> MSANSPTGNDPHVFGIPVNATPSNMGSPGSPVNVPPPMNPAVANVNHPVMRTNSNSNANEGTRTLTREQIQQLQQRQRLLLQQRLLEQQRKQQALQNYEAQFYQMLMTLNKRPKRLYNFVEDADSILKKYEQYLHSFEFHIYENNYKICAPANSRLQQQQKQPELTSDGLILTKNNETLKEFLEYVARGRIPDAIMEVLRDCNIQFYEGNLILQVYDHTNTVDVTPKENKPNLNSSSSPSNNNSTQDNSKIQQPSEPNSGVANTGANTANKKASFKRPRVYRTLLKPNDLTTYYDMMSYADNARFSDSIYQQFESEILTLTKRNLSLSVPLNPYEHRDMLEETAFSEPHWDSEKKSFIHEHRAESTREGTKGVVGHIEERDEFPQHSSNYEQLMLIMNERTTTITNSTFAVSLTKNAMEIASSSSNGVRGASSSTSNSASNTRNNSLANGNQVALAAAAAAAAVGSTMGNDNNQFSRLKFIEQWRINKEKRKQQALSANINPTPFNARISMTAPLTPQQQLLQRQQQALEQQQNGGAMKNANKRSGNNATSNNNNNNNNLDKPKVKRPRKNAKKSESGTPAPKKKRMTKKKQSASSTPSSTTMS;> MSSNPENSGVNANNNTGTGNADAITGAQQNMVLQPRQLQEMAAKFRTLLTEARNVGETTPRGKELMFQAAKIKQVYDALTLNRRRQQAAQAYNNTSNSNSSNPASIPTENVPNSSQQQQQQQQQTRNNSNKFSNMIKQVLTPEENQEYEKLWQNFQVRHTSIKEKETYLKQNIDRLEQEINKQTDEGPKQQLQEKKIELLNDWKVLKIEYTKLFNNYQNSKKTFYVECARHNPALHKFLQESTQQQRVQQQRVQQQQQQQQQQQQQQQQQQQQQQQRQGQNQRKISSSNSTEIPSVTGPDALKSQQQQQNTITATNNPRGNVNTSQTEQSKAKVTNVNATASMLNNISSSKSAIFKQTEPAIPISENISTKTPAPVAYRSNRPTITGGSAMNASALNTPATTKLPPYEMDTQRVMSKRKLRELVKTVGIDEGDGETVIDGDVEELLLDLADDFVTNVTAFSCRLAKHRKSDNLEARDIQLHLERNWNIRIPGYSADEIRSTRKWNPSQNYNQKLQSITSDKVAAAKNNGNNVASLNTKK;> MSLTEQIEQFASRFRDDDATLQSRYSTLSELYDIMELLNSPEDYHFFLQAVIPLLLNQLKEVPISYDAHSPEQKLRNSMLDIFNRCLMNQTFQPYAMEVLEFLLSVLPKENEENGILCMKVLTTLFKSFKSILQDKLDSFIRIIIQIYKNTPNLINQTFYEAGKAEQGDLDSPKEPQADELLDEFSKNDEEKDFPSKQSSTEPRFENSTSSNGLRSSMFSFKILSECPITMVTLYSSYKQLTSTSLPEFTPLIMNLLNIQIKQQQEAREQAESRGEHFTSISTEIINRPAYCDFILAQIKATSFLAYVFIRGYAPEFLQDYVNFVPDLIIRLLQDCPSELSSARKELLHATRHILSTNYKKLF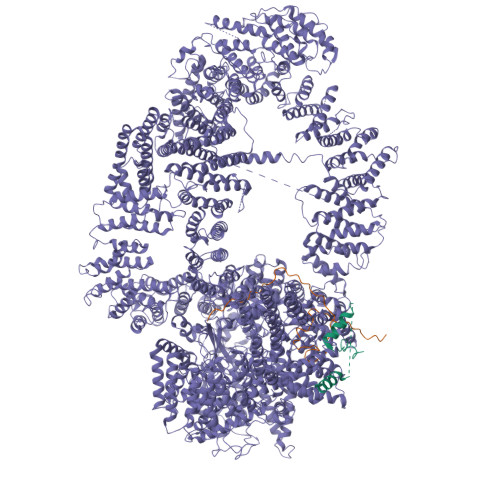LPKLDYLFDERILIGNGFTMHETLRPLAYSTVADFIHNIRSELQLSEIEKTIKIYTGYLLDESLALTVQIMSAKLLLNLVERILKLGKENPQEAPRAKKLLMIIIDSYMNRFKTLNRQYDTIMKYYGRYETHKKEKAEKLKNSIQDNDKESEEFMRKVLEPSDDDHLMPQPKKEDINDSPDVEMTESDKVVKNDVEMFDIKNYAPILLLPTPTNDPIKDAFYLYRTLMSFLKTIIHDLKVFNPPPNEYTVANPKLWASVSRVFSYEEVIVFKDLFHECIIGLKFFKDHNEKLSPETTKKHFDISMPSLPVSATKDARELMDYLAFMFMQMDNATFNEIIEQELPFVYERMLEDSGLLHVAQSFLTSEITSPNFAGILLRFLKGKLKDLGNVDFNTSNVLIRLFKLSFMSVNLFPNINEVVLLPHLNDLILNSLKYSTTAEEPLVYFYLIRTLFRSIGGGRFENLYRSIKPILQVLLQSLNQMILTARLPHERELYVELCITVPVRLSVLAPYLPFLMKPLVFALQQYPDLVSQGLRTLELCIDNLTAEYFDPIIEPVIDDVSKALFNLLQPQPFNHAISHNVVRILGKLGGRNRQFLKPPTDLTEKTELDIDAIADFKINGMPEDVPLSVTPGIQSALNILQSYKSDIHYRKSAYKYLTCVLLLMTKSSAEFPTNYTELLKTAVNSIKLERIGIEKNFDLEPTVNKRDYSNQENLFLRLLESVFYATSIKELKDDAMDLLNNLLDHFCLLQVNTTLLNKRNYNGTFNIDLKNPNFMLDSSLILDAIPFALSYYIPEVREVGVLAYKRIYEKSCLIYGEELALSHSFIPELAKQFIHLCYDETYYNKRGGVLGIKVLIDNVKSSSVFLKKYQYNLANGLLFVLKDTQSEAPSAITDSAEKLLIDLLSITFADVKEEDLGNKVLENTLTDIVCELSNANPKVRNACQKSLHTISNLTGIPIVKLMDHSKQFLLSPIFAKPLRALPFTMQIGNVDAITFCLSLPNTFLTFNEELFRLLQESIVLADAEDESLSTNIQKTTEYSTSEQLVQLRIACIKLLAIALKNEEFATAQQGNIRIRILAVFFKTMLKTSPEIINTTYEALKGSLAENSKLPKELLQNGLKPLLMNLSDHQKLTVPGLDALSKLLELLIAYFKVEIGRKLLDHLTAWCRVEVLDTLFGQDLAEQMPTKIIVSIINIFHLLPPQADMFLNDLLLKVMLLERKLRLQLDSPFRTPLARYLNRFHNPVTEYFKKNMTLRQLVLFMCNIVQRPEAKELAEDFEKELDNFYDFYISNIPKNQVRVVSFFTNMVDLFNTMVITNGDEWLKKKGNMILKLKDMLNLTLKTIKENSFYIDHLQLNQSIAKFQALYLRFTELSERDQNPLLLDFIDFSFSNGIKASYSLKKFIFHNIIASSNKEKQNNFINDATLFVLSDKCLDARIFVLKNVINSTLIYEVATSGSLKSYLVEDKKPKWLELLHNKIWKNSNAILAYDVLDHHDLFRFELLQLSAIFIKADPEIIAEIKKDIIKFCWNFIKLEDTLIKQSAYLVTSYFISKFDFPIKVVTQVFVALLRSSHVEARYLVKQSLDVLTPVLHERMNAAGTPDTWINWVKRVMVENSSSQNNILYQFLISHPDLFFNSRDLFISNIIHHMNKITFMSNSNSDSHTLAIDLASLILYWENKTLEITNVNNTKTDSDGDVVMSDSKSDINPVEADTTAIIVDANNNSPISLHLREACTAFLIRYVCASNHRAIETELGLRAINILSELISDKHWTNVNVKLVYFEKFLIFQDLDSENILYYCMNALDVLYVFFKNKTKEWIMENLPTIQNLLEKCIKSDHHDVQEALQKVLQVIMKAIKAQGVSVIIEEESPGKTFIQMLTSVITQDLQETSSVTAGVTLAWVLFMNFPDNIVPLLTPLMKTFSKLCKDHLSISQPKDAMALEEARITTKLLEKVLYILSLKVSLLGDSRRPFLSTVALLIDHSMDQNFLRKIVNMSRSWIFNTEIFPTVKEKAAILTKMLAFEIRGEPSLSKLFYEIVLKLFDQEHFNNTEITVRMEQPFLVGTRVEDIGIRKRFMTILDNSLERDIKERLYYVIRDQNWEFIADYPWLNQALQLLYGSFNREKELSLKNIYCLSPPSILQEYLPENAEMVTEVNDLELSNFVKGHIASMQGLCRIISSDFIDSLIEIFYQDPKAIHRAWVTLFPQVYKSIPKNEKYGFVRSIITLLSKPYHTRQISSRTNVINMLLDSISKIESLELPPHLVKYLAISYNAWYQSINILESIQSNTSIDNTKIIEANEDALLELYVNLQEEDMFYGLWRRRAKYTETNIGLSYEQIGLWDKAQQLYEVAQVKARSGALPYSQSEYALWEDNWIQCAEKLQHWDVLTELAKHEGFTDLLLECGWRVADWNSDRDALEQSVKSVMDVPTPRRQMFKTFLALQNFAESRKGDQEVRKLCDEGIQLSLIKWVSLPIRYTPAHKWLLHGFQQYMEFLEATQIYANLHTTTVQNLDSKAQEIKRILQAWRDRLPNTWDDVNMWNDLVTWRQHAFQVINNAYLPLIPALQQSNSNSNINTHAYRGYHEIAWVINRFAHVARKHNMPDVCISQLARIYTLPNIEIQEAFLKLREQAKCHYQNMNELTTGLDVISNTNLVYFGTVQKAEFFTLKGMFLSKLRAYEEANQAFATAVQIDLNLAKAWAQWGFFNDRRLSEEPNNISFASNAISCYLQAAGLYKNSKIRELLCRILWLISIDDASGMLTNAFDSFRGEIPVWYWITFIPQLLTSLSHKEANMVRHILIRIAKSYPQALHFQLRTTKEDFAVIQRQTMAVMGDKPDTNDRNGRRQPWEYLQELNNILKTAYPLLALSLESLVAQINDRFKSTTDEDLFRLINVLLIDGTLNYNRLPFPRKNPKLPENTEKNLVKFSTTLLAPYIRPKFNADFIDNKPDYETYIKRLRYWRRRLENKLDRASKKENLEVLCPHLSNFHHQKFEDIEIPGQYLLNKDNNVHFIKIARFLPTVDFVRGTHSSYRRLMIRGHDGSVHSFAVQYPAVRHSRREERMFQLYRLFNKSLSKNVETRRRSIQFNLPIAIPLSPQVRIMNDSVSFTTLHEIHNEFCKKKGFDPDDIQDFMADKLNAAHDDALPAPDMTILKVEIFNSIQTMFVPSNVLKDHFTSLFTQFEDFWLFRKQFASQYSSFVFMSYMMMINNRTPHKIHVDKTSGNVFTLEMLPSRFPYERVKPLLKNHDLSLPPDSPIFHNNEPVPFRLTPNIQSLIGDSALEGIFAVNLFTISRALIEPDNELNTYLALFIRDEIISWFSNLHRPIIENPQLREMVQTNVDLIIRKVAQLGHLNSTPTVTTQFILDCIGSAVSPRNLARTDVNFMPWF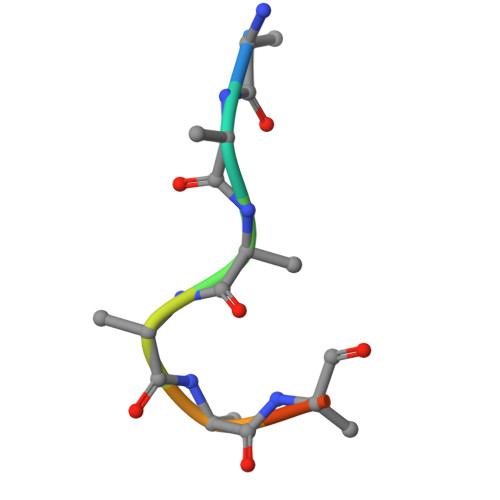> SYSMEHFR> GSLELELQNLELLVHIAEVLARLARRTGNEEALEHAARVAEEVAKQAEEIAREARYRGDLRLALEALRIMVEAARVLAEIARERGNEELLQKAEELA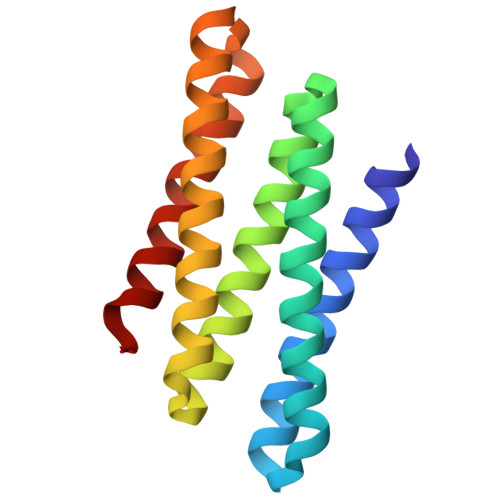REALRQVREISKRLQEEGNIELALKANRLLIDALEVLVRIMRHR> NNSQLVVSVAGTVEGTNQDISLKFFEID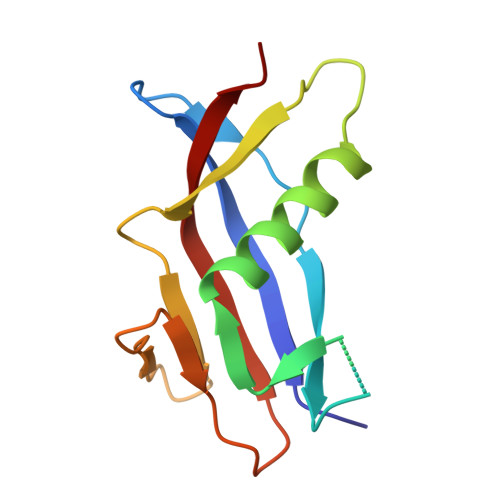LTSRPASKPFATDSGAMPHKLEKADLLKAIQEQLIANVHSNDDYFEVIDFASDATITDRNGKVYFADKDGSVTLPTQPVQEFLLSGHVRVRPYK> INLSNKTDENTISFFDSGDPERMNSEALMRGCGEQIVNLRPLLRTFRTINDNWSLAANTKTPITDLTNTADAEGRDYMSYLSFLYRFYRGGRRYKFFNTTPLKQSQTCYVRSFLIPRNYTADEINTDGPSHITYPVINPVHEVEVPFYSQYRKIPIASTTDKGYDSSLMYYTNVGTQQIVARAGNDDFTFGWMIGTPQLQGITKEVAN;> NVHNTK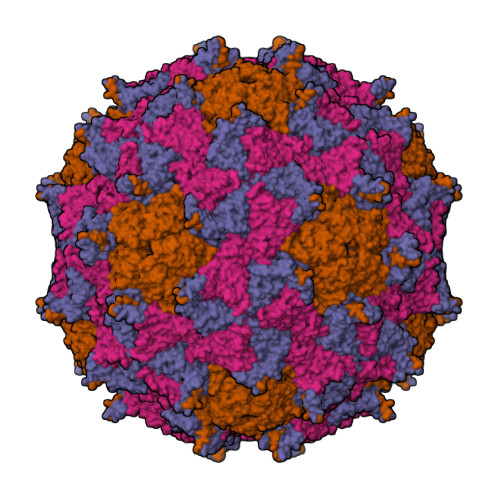LASTSAENAIEKEQITTFHDVETPNRIDTPMAQDTSSARSMDDTHSIIQFLQRPVLIDNIEIVAGTTADNNTALSRYVLDRTNPQKYIKQWTLPSTVLKAGGKAQKLANFKYLRCDVQVKLVLNANPFIAGRLYLAYSPYDDKVAPERRIIYTSRAGVTGYPGVELDFQLDNSVEMTIPYASFQEAYDLVSGNEDFVQLYLFTIAPVLGPSAESANSKVDLSVYMWLDNISLVIPTYRLNPNL;> SKPRNQNQVMPLQNVPGWGYSLYKGIDMSVPLAYDPNNELGDLRDVFPSAVDEMAIGYVCGNPAIKHVLTWSTTDVVQNPISNGDDWGGVIPVGMPCYSKTIRAVKGATSTKTEVMDPAPCEYVANLFSYWRATMCYRITVVKTAFHTGRLEIFFEPGSIPTVRTADNLGPDQTQLNGTIAPSDNNYKYILDLTNDTEVTIKVPYVSNKMFMKTVGIYGAHDEDNWNFDESFTGFLCIRPITKLMAPDTVSQKVSIVVWKWAEDVVVVEPKPLTSGPTQVYNPPAVARDL;> PTSENPKIGPISEVASGVKTAANGIERIPVLGEIAKPVTAAVKWFADIVGGVAAIFGW>[2x]GCGXGCG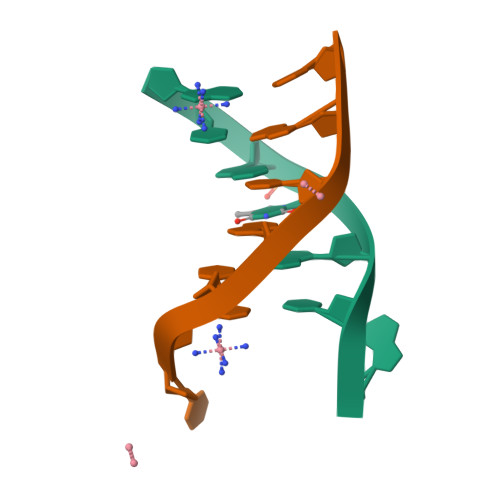;>[2x]CGCACGC> YRVQPSGKGGL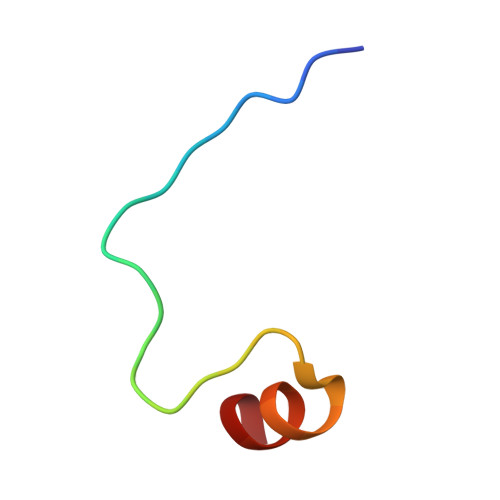RPGVDLSSNAALAEAMN> MYTNSDFVVIKALEDGVNVIGLTRGADTRFHHSEKLDKGEVLIAQFTEHTSAIKVRG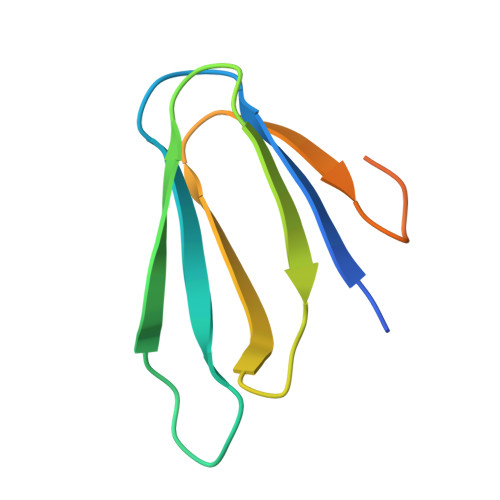KAYIQTRHGVIESEGKKAAAAAAA>[2x]MAHHHHHHMDAATTRAGLTDLKFRLVRESFADAVSWVAKNLPTRPAVPVLSGVLLTGSDEGLTISGFDYEVSAEVRVPAEIASPGTVLVSGR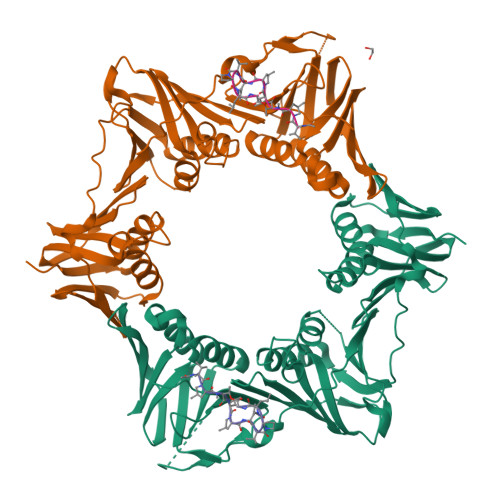LLSDITRALPNKPVDFYVDGNRVALTCGNARFSLPTMAVEDYPTLPTLPEDTGTLPAELFSEAIGQVAIAAGRDDTLPMLTGIRVEISGEKVVLAATDRFRLAVRELTWNALSPDIEAAVLVPAKTLGEAAKANTDGSEVRLSLGAGMGVGKDGLLGISGDGKRSTTRLLDAEFPKFRQLLPAEHTAVASADVAELTEAIKLVALVADRGAQVRMEFADGMLRLSAGADDVGRAEEDIAVEFAGQPLTIAFNPTYLIDGLASLHSERVSFGFTTPGKPALLRPASAEDRIVSGPGDQGPFAAVPTDYVYLLMPVRLPG;>XVPTLPLVPXG[2x]>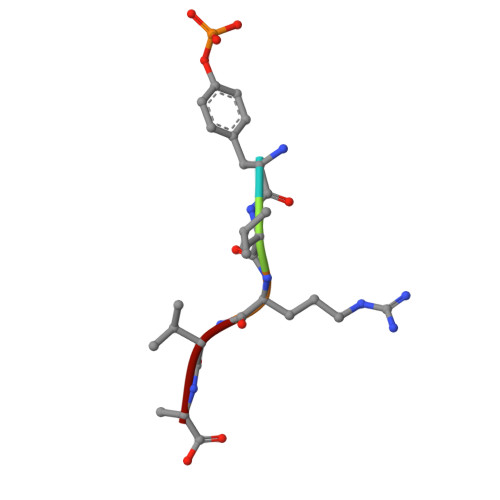 YLRVA>[3x]MSLADHLTELRSRLMRATIAVLILGTI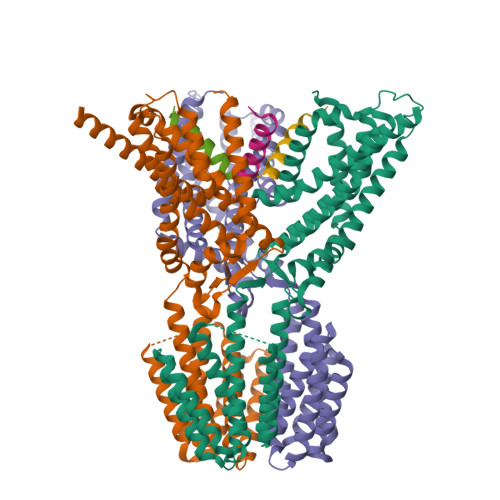SLVFAKPIFGLLMQPVLDALPPENRSLIYTSGIEELNVLMKVGVYAGIFLTTPVILMQIWGFVSPGLYPEERRFAAPFVAFGSIAFLLGAAFAYFAVLPSMFTFLLNEEETLALEQRLDTARLRADDALRFLRLGEAEEAGRIAKETSTQLRAEGQGQAPAPEVAPAASVEMTGRLDGLGRLLDAASVGYGAQSRGVLRQAVEKRVEAVTAYEKKDFAAAAAAMDGSASLLAGIAPTRTEELAGLWRLEKELATAHAAHEAARWTRPMLSMHEQLSLVLLLILAFGIIFELPLVMALLGVVGVVKSSWLFRYQRHAFVVALIAAAIITPTGDVVNLSLMAGPMLLAYELGVLLVWMVERRRARNSAETGITPASGSENLYFQ;>[3x]MFNIGAGEMVFILVAALLILGPQRLPELARGIGKFLREFRRQTDEVRNVVEREFYAMDQEIGEPPTAPLRPGTRFAPQPPQAVGGPEATLPPATDGASPPADAASPQPSSPAQVLEMDAQGPREVATSDVHAGETPAQDAATAEPGAEPTAEAPPEPAASTATSPTLSPIPGTVARNAPKRSWSHPQFEK> GSHMSRDMSSTAQRLKFLDEGVEEIDIELARLRFESAVETLLDIESQLEDLSERISDEELMLLNLISLKIEQRREAISSKLSQSILSSNEIVHLKSGTENMIKLGLPEQALDLFLQNRSNFIQDLILQIGSVDNPTN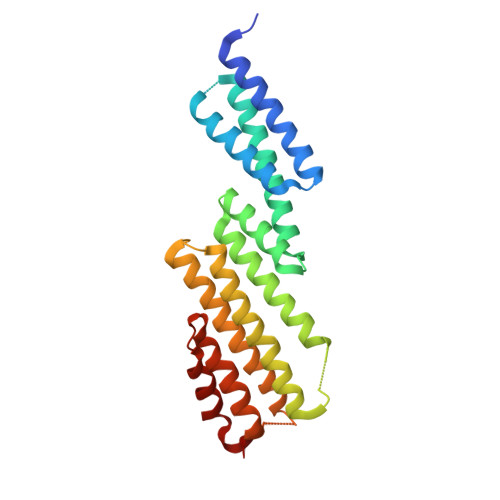YLTQLAVIRFQTIKKTVEDFQDIFKELGAKISSILVDWCSDEVDNHFKLIDKQLLNDEMLSPGSIKSSRKQIDGLKAVGLDFVYKLDEFIKKNSDKIR> MQNEKLDHESVTQAMQPKDTPELRALYKSFEEESIIPLWTQLGDLMPIHPKSKAVPHVWKWSTLLRLARKSGELVPVGRGGERRALGLANPGLGGNAYISPTMWAGIQYLGPRE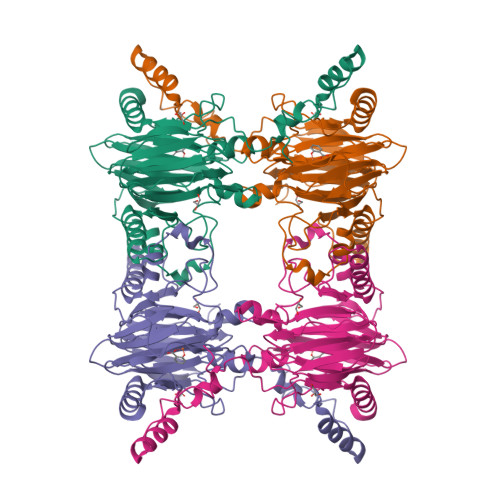TAPEHRHSQNAFRFVVEGEGVWTVVNGDPVRMSRGDLLLTPGWCFHGHMNDTDQPMAWIDGLDIPFSQQMDVGFFEFGSDRVTDYATPNFSRGERLWCHPGLRPLSGLQNTVASPIGAYRWEFTDRALTEQLLLEDEGQPATVAPGHAAIRYVNPTTGGDVMPTLRCEFHRLRAGTETATRNEVGSTVFQVFEGAGAVVMNGETTKLEKGDMFVVPSWVPWSLQAETQFDLFRFSDAPIMEALSFMRTKIEGQK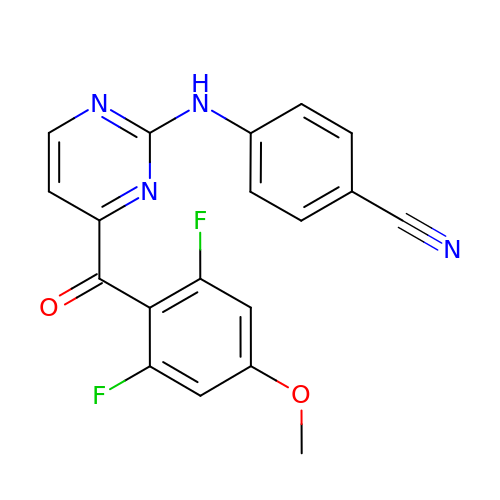4-{[4-(2,6-difluoro-4-methoxybenzene-1-carbonyl)pyrimidin-2-yl]amino}benzonitrile | C19 H12 F2 N4 O2 | FZZMKUKEMAVUGK-UHFFFAOYSA-N> MRSRRV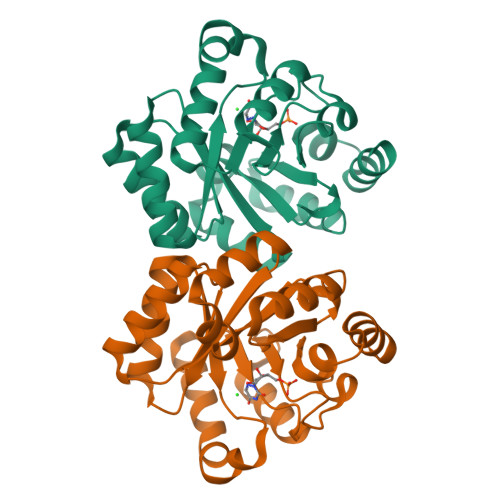DVMDVMNRLILAMDLMNRDDALRVTGEVREYIDTVKIGYPLVLSEGMDIIAEFRKRFGCRIIADFKVANIPETNEKICRATFKAGADAIIVHGFPGADSVRACLNVAEEMGREVFLLTEMSHPGAEMFIQGAADEIARMGVDLGVKNYVGPSTRPERLSRLREIIGQDSFLISPGVGAQGGDPGETLRFADAIIVGRSIYLADNPAAAAAGIIESIKDLLIPEDPAANKARKEAELAAATA>TTGGGCCGAA[2x];>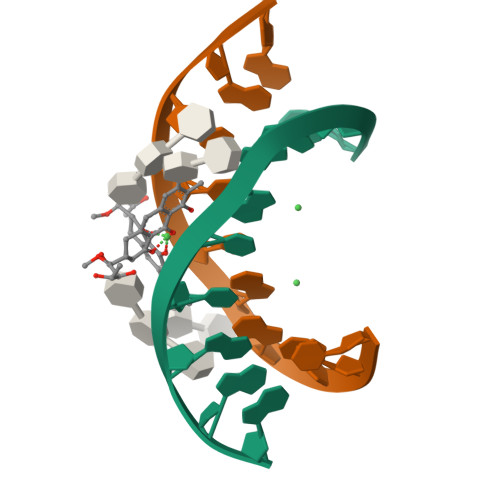TTCGGCCCAA[2x]> LGTNYLLSGQTLNTDGHLKNGDFDLVMQN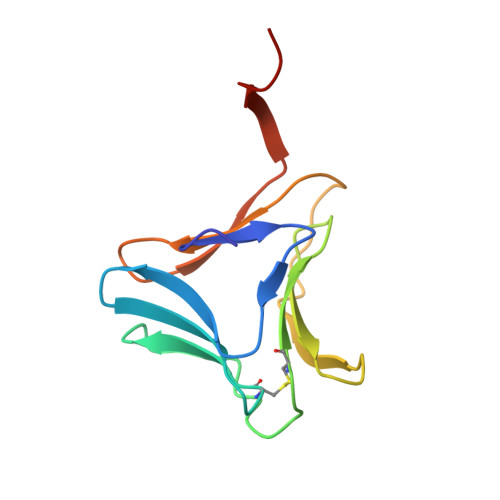DCNLVLYNGNWQSNTANNGRDCKLTLTDYGELVIKNGDGSTVWRSRAKSVKGNYAAVLHPDGRLVVFGPSVFKIDPWVPGL Therefore, oligoribonucleases (ORN), RNases targeted toward short oligonucleotides, are needed for the complete digestion of short oligonucleotides into mononucleotides. Among these, ORN belongs to the DEDD superfamily, comprising 3′-5′ exonucleases that require a divalent cation for activity. Our research group have focused on the mechanism of action of oligoribonuclease (CpsORN) from the psychrophilic gram-negative bacterium Colwellia psychrerythraea strain 34H, to understand how the enzyme hydrolyses small nucleic acids. Structural analysis results show that CpsORN is a stable dimer and its active site is formed by swapping residues from the other subunit.

In the two linked uridine (U-U)-bound structure, sufficient electron density was observed for only two uridine molecules, although five linked uridine (5′-U(-3)-U(-2)-U(-1)-U(1)-U(2)-3′) was used for crystallisation. Even though a partial electron density of the third uridine was observed, the intensity of electron density was significantly weak. This means that CpsORN tightly grabs only the last two nucleotides of the 5-mer RNA. Meanwhile, the rest of the 5-mer RNA are located outside the binding pocket, in a flexible state. For this RNA-bound structure determination, D163A inactive mutant CpsORN protein was used, as mentioned in the pNP-TMP-bound structure. The last two ribonucleotides make hydrophobic stacking interactions with Leu18, Trp61, and Tyr129 residues. A more detailed examination revealed that the indole ring of Trp61 forms a hydrophobic interaction with the base of nucleotide U2, forming a barrier at the end of the bound RNA substrate. The side chain of Leu18 is located between the bases of nucleotides U1 and U2 of the bound substrate. The phenyl ring of Tyr129 forms a hydrophobic interaction with the base of nucleotide U1. All these interacting residues act as a wedge that may allow CpsORN to cleave the exact position of RNA substrate and guide the 3′-terminal exo-RNA cutting.

>[2x]MAGNDSNLIWLDLEMTGLEPVEDVILEIAIIITDSELNILAQGPIFAISQTDDVLDNMNPWCIEHHGKSGLTQRCRDSEVSLAHATKESLAFVQEWVPQGKSPMCGNSIGQDRRFINKYMPDFEDHFHYRNLDVSTIKELAKRWKPEVLESVVKTGAHLALDAIKESIAELKVYRELFFKL>[4x]SDPTPDQMEGPYFKPDSPPRTSLVTSSTPGVPLTVSGYVFGRACKPLTGVLLDFWQADTGGAYD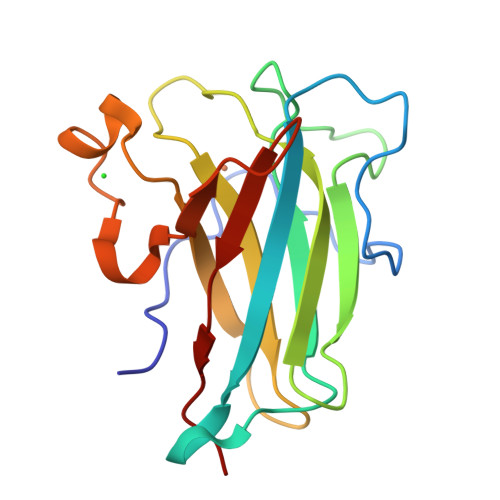MTGFAFRGHQFTGADGSFTLRTIVPGLYPGRTRHIHVKAQAPGRPVLTTQLYFPGEPRNTTDALFDPALLMNVRSAGPGREGTFDFVLDVA> MTTTERPDLAWLDEVTMTQLERNPYEVYERLRAEAPLAFVPVLGSYVASTAEVCREVATSPDFEAVITPAGGRTFGHPAIIGVNGDIHADLRSMVEPALQPAEVDRWIDDLVRPIARRYLERFENDGHAELVAQYCEPVSVRSLGDLLGLQEVDSDKLREWFAKLNRSLTNAAVDENGEFANPEGFAEGDQAKAEIRAVVDPLIDKWIEHPDDSAISHWLHDGMPPGQTRDREYIYPTIYVYLLGAMQEPGHGMASTLVGLFSRPEQLEEVVDDPTLIPRAIAEGLRWTSPIWSATARISTKPVTIAGVDLPAGTPVMLSYGSANHDTGKYEAPSQYDLHRPPLPHLAFGAGNHACAGIYFANHVMRIALEELFEAIPNLERDTREGVEFWGWGFRGPTSLHVTWEV

GcoA belongs to the CYP255A family of cytochrome P450 enzymes. Our recent characterization of a two-component P450 enzyme system consisting of a reductase, GcoB, and a P450 oxidase, GcoA, demonstrated that it demethylates diverse aromatic compounds, including guaiacol (which can be derived from coniferyl alcohol and represents the aromatic functionality of G-lignin that must undergo demethylation), guaethol, anisole (methoxybenzene), 2-methylanisole, and 3-methoxycatechol (3MC) with similar or greater efficiency than other O-aryl-demethylases described in the literature. However, GcoAB shows poor reactivity toward syringol, which can be derived from sinapyl alcohol via high-temperature reactions and represents the aromatic functionality of S-lignin that must undergo O-demethylation for further catabolism via ring-opening dioxygenases. In the present study, we hypothesized that substitution of GcoA-F169, which has the closest interaction with the bound substrate, may relax the specificity of the enzyme sufficiently to permit the O-demethylation of S-lignin type substrates.

The closest contact is with GcoA-F169, which forms a hydrophobic interaction with the C6 carbon on the aromatic ring of guaiacol. A broader survey of variants at the GcoA-F169 position (amino acids S, H, V, I, and L in addition to A) confirmed that GcoA-F169A exhibits the best catalytic performance in terms of both specific activity and reaction coupling, although other small side chains (S and V) also permitted reactivity with syringol, suggesting that these may permit syringol to assume a reactive conformation at the heme. Each protein variant also crystallized successfully with guaiacol and the structures showed that the orientation of the bound ligand remained consistent with that of the WT enzyme. Furthermore, comparison of the surrounding active site architecture confirmed no significant deviation from the WT.>[2x]GPGSMPHPSLKSNRALPLLTFARTHSFAIPAICVYNLEGILAIIRAAEHKRSPAMILLFPWAIQYADSLLVRTAASACRAASVPITLHLDHAQDPEIIKRAADLSRSETHEPGFDSIMVDMSHFSKEENLRLTRELVAYCNARGIATEAEPGRIEG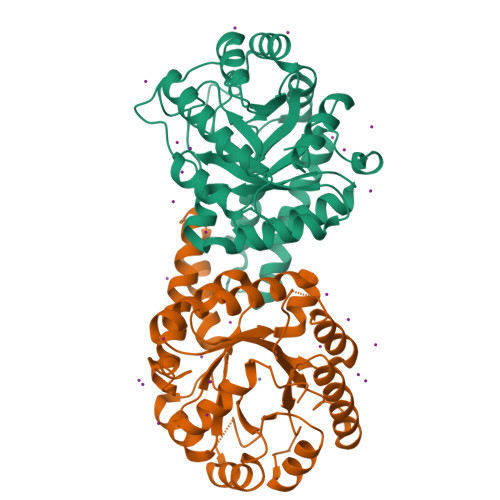GEDGVQDTVDLEGVLTTPEESEEFVATGINWLAPAFGNVHGNYGPRGVQLDYERLQRINEAVGERVGLVLHGADPFTKEIFEKCIERGVAKVNVNRAVNNEYVKVMREKAGSLPITRLHEEVTNAMQAAVEKIMDMIDSTGKAEFMMDEK> MQQKLENIKFVITDVDGVLTDGQLHYDANGEAIKSFHVRDGLGIKMLMDADIQVAVLSGRDSPILRRRIADLG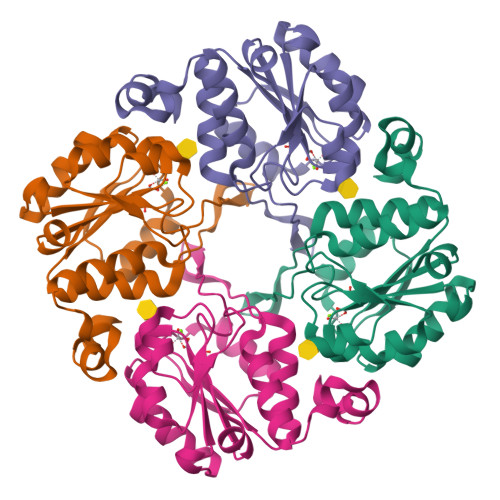IKLFFLGKLEKETACFDLMKQAGVTAEQTAYIGDDSVDLPAFAACGTSFAVADAPIYVKNAVDHVLSTHGGKGAFREMSDMILQAQGKSSVFDTAQGFLKSVKSMGQ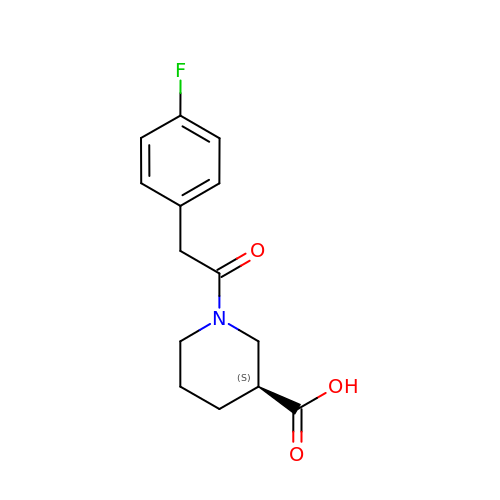(3S)-1-[(4-fluorophenyl)acetyl]piperidine-3-carboxylic acid | C14 H16 F N O3 | ISRBHDOSFNPUED-UHFFFAOYSA-N>STLKGALSVKFDVKCPADKFFSAFVEDTNRPFEKNGKTEIEAVDLVKKTMTIQMSGSEIQKYFKTLKGSIAVTPIGVGDGSHVVWTFHFEKVHKDIDDPHSIIDESVKYFKKLDEAILNFKE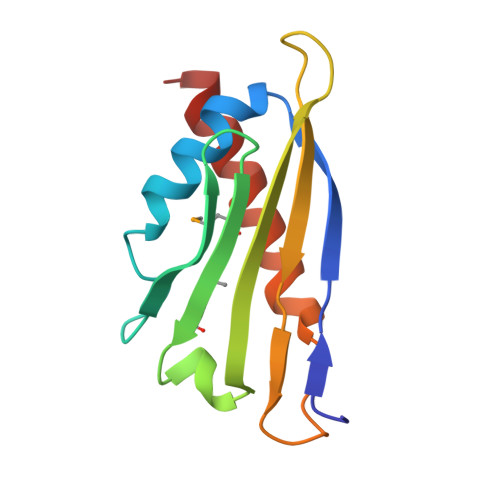[2x]>GHMTGAHERTFLAVKPDGVQRRLVGEIVRRFERKGFKLVALKLVQASEELLREHYAELRERPFYGRLVKYMASGPVVAMVWQGLDVVRTSRALIGATNPADAPPGTIRGDFCIEVGKNLIHGSDSVESARREIALWFRADELLCWEDSAGHWLYE[6x]

With regard to their common enzymatic activity, NDPKs are NTP/NDP transphosphorylases encoded by the nme genes. They catalyze the transfer of the γ-phosphate group from an NTP to an NDP via the formation of a high-energy intermediate on a catalytic histidine residue. We produced a truncated version of human NDPK isoform C (residues Thr18–Glu169, NDPK-C hereafter) and determined the 3D structure via X-ray crystallography in the absence and presence of various nucleotides. A data analysis revealed a hexameric arrangement, which is organized as three dimers, as previously reported for other functional eukaryotic NDPK variants.

Crystals of NDPK-C in a complex with ADP grew in two different conditions: (1) in a metal chelating screening solution containing citrate (see the Methods section), we obtained crystals without the magnesium ion; and (2) under non-chelating crystallization conditions, a magnesium ion was detected in the active site. The magnesium-containing crystals (belonging to space group C2) diffracted to a resolution of 2.10 Å. Essentially, we detected a very similar mode of nucleotide binding including the residues described above for the metal ion free form (Phe77, Val129, Asn132, Lys29, Arg105 and Thr111). Arg122 showed the same position and orientation, but its contact to the β-phosphate of ADP was lost as evidenced by a change in the distance from 2.9 to 4 Å. In addition to the residues already described (Tyr69, His135 and Gly136), Asp138 was also part of the pocket, and we observed four water molecules which localized in a square pyramidal manner around the metal ion; the fifth coordination site was occupied by an oxygen from the nucleotide α-phosphate. However, a superposition of the nucleotide-binding pockets in the absence and presence of magnesium revealed that the magnesium ion induces a change in the conformation of the phosphate groups with the consequence of a weakened connection of ADP to Arg122. Thus, the magnesium ion changed the number, localization and coordination of the water molecules as well as the conformation of the nucleotide phosphate chain. In our NDPK-C structure, we observed the same coordination of Mg2+ to three water molecules and the α- and β-phosphate of ADP. First of all, these data indicate that we crystallized an active form of human NDPK-C in complex with ADP and Mg2+ in the C2 space group. During catalysis, the Mg2+ is indispensable in stabilizing the negative charge of the leaving phosphate from ATP at the transition state.>[5x]TITLEKKVRKGIESLITELKLMQAVLSKVSKVPADQLDEGVKIWAGNVKELSYQMEDIVDAFMVRVGDGGESTNPKNRVKKILKKVKKLFKNGKDLHRISAALEEVVLQAKQLAELRQRYEQEMRDTSAQTSVDPRMMALYTDVTELVGIEETRDKLINMLTEGDDWSKHPLKTISIVGFGGLGKTTLAKAAYDKIKVQFDCGAFVSVSRNPEMKKVLKDILYGLDKVKYENIHNAARDEKYLIDDIIEFLNDKRYLIVIDDIWNEKAWELIKCAFSKKSPGSRLITTTRNVSVSEACCSSEDDIYRMEPLSNDVSRTLFCKRIFSQEEGCPQELLKVSEEILKKCGGVPLAIITIASLLANKGHIKAKDEWYALLSSIGHGLTKNRSLEQMKKILLFSYYDLPSYLKPCLLYLSIFPEDREIRRARLVWRWISEGFVYSEKQDISLYELGDSYFNELVNRSMIQPIGIDDEGKVKACRVHDMVLDLICSLSSEENFVTILDDPRRKMPNSESKVRRLSIQNSKIDVDTTRMEHMRSVTVFSDNVVGKVLDISRFKVLRVLDLEGCHVSDVGYVGNLLHLRYLGLKGTHVKDLPMEVGKLQFLLTLDLRGTKIEVLPWSVVQLRRLMCLYVDY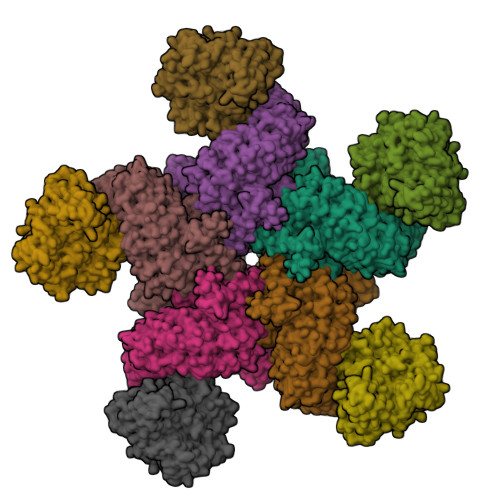GMKLPSGIGNLTFLEVLDDLGLSDVDLDFVKELGRLTKLRVLRLDFHGFDQSMGKALEESISNMYKLDSLDVFVNRGLINCLSEHWVPPPRLCRLAFPSKRSWFKTLPSWINPSSLPLLSYLDITLFEVRSEDIQLLGTLPALVYLEIWNYSVFEEAHEVEAPVLSSGAALFPCATECRFIGIGAVPSMFPQGAAPRLKRLWFTFPAKWSSSENIGLGMRHLPSLQRVVVDVISEGASREEADEAEAALRAAAEDHPNRPILDIW;>[5x]VNFPFPKKMITESNSKDIREYLASTFPFEQQSTILDSVKSIAKVQIDDRKAFDLQLKFRQENLAELKDQIILSLGANNGNQNWQKLLDYTNKLDELSNTKISPEEFIEEIQKVLYKVKLESTSTSKLYSQFNLSIQDFALQIIHSKYKSNQISQNDLLKLITEDEMLKILAKTKVLTYKMKYFDSASKMGINKYISTEMMDLDWQFSHYKTFNDALKKNKASDSSYLGWLTHGYSIKYGLSPNNERSMFFQDGRKYAELYAFSKSPHRKIIPGEHLKDLLAKINKSKGIFLDQNALLDKRIYAFHELNTLETHFPGITSSFTDDLKSNYRKKMESVSLTCQVLQEIGNIHRFIESKVPYHSSTEYGLFSIPKIFSIPIDYKHGEKENLVSYVDFLYSTAHERILQDNSINQLCLDPLQESLNRIKSNIPVFFNL> MGPSLDFALSLLRRNIRQVQTDQGHFTMLGVRDRLAVLPRHSQPGKTIWVEHKLINILDAVELVDEQGVNLELTLVTLDTNEKFRDITKFIPENISAASDATLVINTEHMPSMFVPVG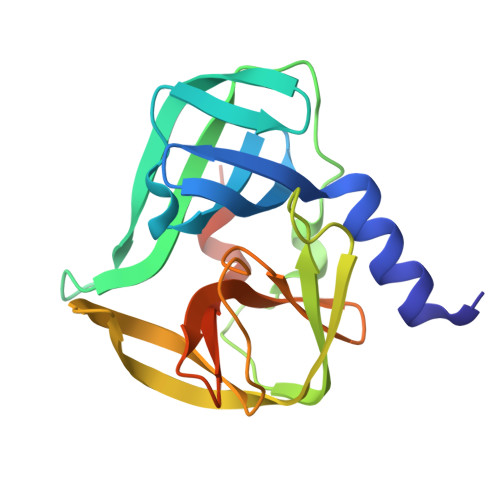DVVQYGFLNLSGKPTHRTMMYNFPTKAGQCGGVVTSVGKVIGIHIGGNGRQGFCAGLKRSYFASEQLEHHHHHH2-(2-QUINOLIN-3-YLPYRIDIN-4-YL)-1,5,6,7-TETRAHYDRO-4H-PYRROLO[3,2-C]PYRIDIN-4-ONE | C21 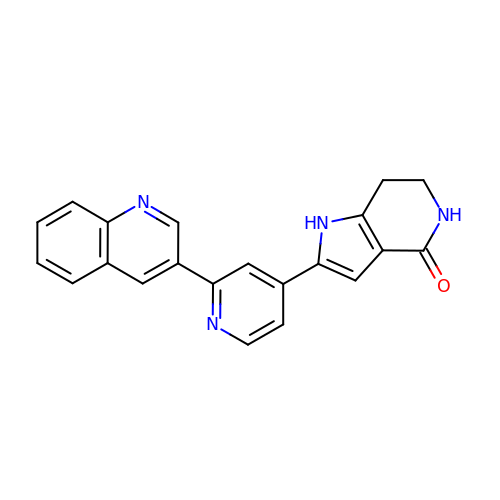H16 N4 O | OWFLADWRSCINST-UHFFFAOYSA-N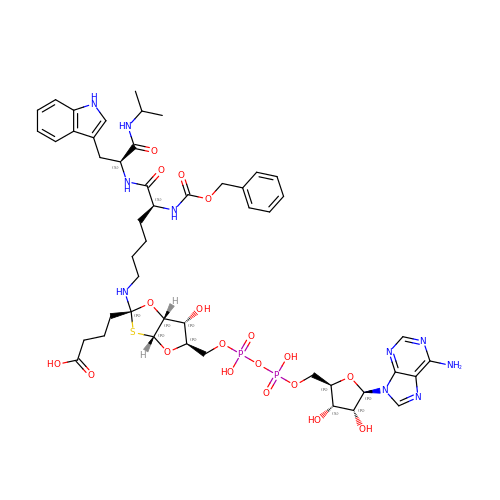4-[(2~{R},3~{a}~{R},5~{R},6~{R},6~{a}~{R})-5-[[[[(2~{R},3~{S},4~{R},5~{R})-5-(6-aminopurin-9-yl)-3,4-bis(oxidanyl)oxolan-2-yl]methoxy-oxidanyl-phosphoryl]oxy-oxidanyl-phosphoryl]oxymethyl]-2-[[(5~{S})-6-[[(2~{S})-3-(1~{H}-indol-3-yl)-1-oxidanylidene-1-(propan-2-ylamino)propan-2-yl]amino]-6-oxidanylidene-5-(phenylmethoxycarbonylamino)hexyl]amino]-6-oxidanyl-3~{a},5,6,6~{a}-tetrahydrofuro[2,3-d][1,3]oxathiol-2-yl]butanoic acid | C48 H64 N10 O19 P2 S | XUCUAEBJCFCJBU-KVSCZEPFSA-N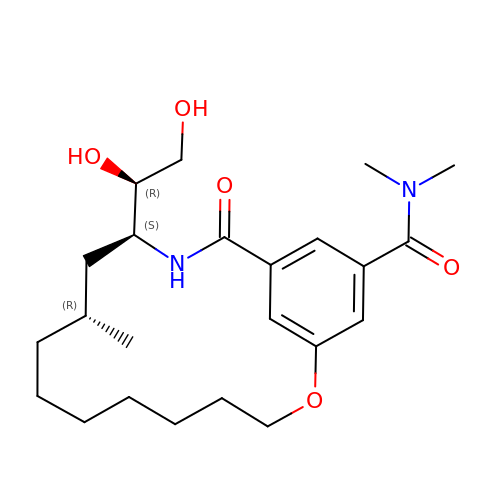(10R,12S)-12-[(1R)-1,2-dihydroxyethyl]-N,N,10-trimethyl-14-oxo-2-oxa-13-azabicyclo[13.3.1]nonadeca-1(19),15,17-triene-17-carboxamide | C23 H36 N2 O5 | FIDGRIKGIUHGAW-CZAAIQMYSA-N>GTSTQTKAGSLTIVGTGIESIGQMTLQALSYIEAAAKVFYCVIDPATEAFILTKNKNCVDLYQYYDNGKSRLNTYTQMSELMVREVRKGLDVVGVFYGHPGVFVNPSHRALAIAKSEGYRARMLPGVSAEDCLFADLCIDPSNPGCLTYEASDFLIRDRPVSIHSHLVLFQVGCVGIADFNFTGFDNNKFGVLVDRLEQEYGAEHPVVHYIAAMMPHQDPVTDKYTVAQLREPEIAKRVGGVSTFYIPPKARKASNLDIIRRLELLPAGQVPDKKARIYPANQWEPDVPEVEPYRPSDQAAIAQLADHAPPEQYQPLATSKAMSDVMTKLALDPKALADYKADHRAFAQSVPDLTPQERAALELGDSWAIRCAMKNMPSSLLDAARESGEEASQNGFP[2x]

While chemical methylation of an amide bond uses a strong base to generate the imidate, OphA, the precursor protein of the fungal peptide macrocycle omphalotin A, self-hypermethylates amides at pH 7 using S-adenosyl methionine (SAM) as cofactor. Omphalotin A derives from the C terminus of the OphA protein, and it is the OphA protein that methylates its own C terminus using S-adenosyl methionine (SAM). The structure of OphA reveals a complex catenane-like arrangement in which the peptide substrate is clamped with its amide nitrogen aligned for nucleophilic attack on the methyl group of SAM. Here, we report the structure of the peptide amide methyltransferase OphA including complexes with cofactor [SAM and S-adenosyl homocysteine (SAH)], cofactor analog, substrate, and product.

The full-length native protein was refractory to crystallization, but an 18-residue C-terminally truncated variant (OphAΔC18), which lacks the sequence that is methylated, was first purified, crystallized, and phased using a selenomethionine variant. Structures with SAM and SAH bound were determined by preincubating the protein with the cofactor prior to crystallization; high-performance liquid chromatography (HPLC) was used to confirm bound cofactor identity. Apart from the addition of the methyl group, the structures of the two complexes are identical [root mean square deviation (rmsd) of 0.6 Å over 684 Cα atoms]. Even with prolonged dialysis at 25°C in the presence of 2 M urea, we were unable to remove SAM from OphAΔC18 to generate an apoprotein (4 M urea unfolded the protein that we were unable to refold). Compared to the Pro242-adenosine (of SAM) interaction in UIIIMT (which binds SAM very tightly), OphAΔC18 makes more extensive van der Waal interactions between Val243 and adenosine. The C-terminal region (Ala252 to Met378) of OphAΔC18, referred to as clasp domain hereafter, is not found in other methyltransferases and comprises extended strands and a helical bundle (Lys322 to Met378). The monomer has the appearance of a ring, with the C-terminal domain forming a thin band, which is closed by interactions between Leu333 and Pro335 from the clasp domain with Leu27 and Ser31 from the N terminus. The clasp domain of one OphAΔC18 monomer wraps around the N-terminal domain of the other monomer, giving the dimer the appearance of two interlocked rings (catenane), a structure that is rare among proteins [reviewed in (20)]. The location of the cofactor relative to the protein is identical in both the OphAΔC18 and OphAΔC6 complexes. Superposition of both sinefungin complexes with the OphAΔC6 Y63F-SAH, OphAΔC18-SAM, and OphAΔC18-SAH complexes shows similar consistency in the protein structure, cofactor, and where present substrate positions.PII-family proteins are key players in the regulation of nitrogen metabolism in bacteria, archaea and in the plastids of plant/algae. All PII proteins known so far show a typical homotrimeric organization. The monomeric unit, of circa 11–18 kDa, consists of two α-helices, four β-strands (organized in a double ferredoxin-like fold β1α1β2β3α2β4) and three protruding loops called B, C and T. In the trimeric state, clefts are formed at the dimeric interface through the interaction of the B-loop and the base of the T-loop of one subunit with the C-loop of the adjacent one. These clefts constitute the binding site for ADP/ATP, magnesium (Mg) and 2OG.

To evaluate the C-terminal extension’s effect on ligand binding, MjGlnK1 was produced and crystallized without a tag. The MtGlnK2 and MjGlnK1woT crystals with Mg-ATP/2OG belonging to tetragonal and rhombohedral forms diffracted to an almost atomic resolution of 1.16 Å and 1.20 Å, respectively. MtGlnK2 and MjGlnK1woT structures, co-crystallized with Mg-ATP and 2OG, offered a very clear picture of the ligand coordination due to their very high-resolution (see Section 4.6). Both structures show an almost identical coordination of the ligands. As expected, the T-loop is drastically switching position between the MtGlnK1-dADP and the ternary complex structure from MtGlnK2-Mg-ATP/2OG and MjGlnK1woT-Mg-ATP/2OG, with a maximum deviation of 11.3 Å and 10.7 Å, respectively (measured at the Cα of the Arg47). In MjGlnK1woT, the carboxy-terminus is coordinating the adenine ring and the Lys90, the latter adequately engages a salt bridge with the β-phosphate of the ATP. The carboxy-terminus is itself locked by the side chain of the Ile via hydrophobic interaction. Therefore, we propose that the absence of the carboxy-terminal provokes a slight displacement of the Lys90 that shifts the coordination of the β-phosphate group. Moreover, the addition of the poly-histidine tag displaces the Mg which cannot bind the 2OG anymore. The results described here point out that the unconventional behavior observed in M. jannaschii is most likely due to the C-terminal His-tag of the MjGlnK1 construct.

> MKKVEAIIRPEKLEIVKKALSDAGYVGMTVSEVKGRGVQGGIVERYRGREYIVDLIPKVKIELVVKEEDVDNVIDIICENARTGNPGDGKIFVIPVERVVRVRTKEEGKEAL> SNISRQAYADMFGPTVGDKVRLADTELWIEVEDDLTTYGEEVKFGGGKVIRDGMGQGQMLAADCVDLVLTNALIVDHWGIVKADIGVKDGRIFAIGKAGNPDIQPNVTIPIGAATEVIAAEGKIVTAGG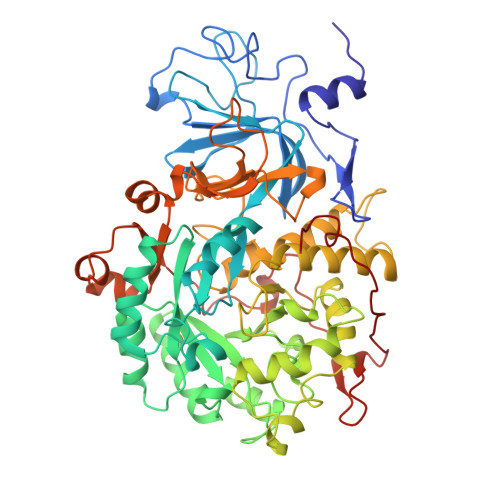IDTHIHWICPQQAEEALVSGVTTMVGGGTGPAAGTHATTCTPGPWYISRMLQAADSLPVNIGLLGKGNVSQPDALREQVAAGVIGLEIHEDWGATPAAIDCALTVADEMDIQVALHSDTLNESGFVEDTLAAIGGRTIHTFHTEGAGGGHAPDIITACAHPNILPSSTNPTLPYTLNTIDEHLDMLMVCHHLDPDIAEDVAFAESRIRRETIAAEDVLHDLGAFSLTSSDSQAMGRVGEVILRTWQVAHRMKVQRGALAEETGDNDNFRVKRYIAKYTINPALTHGIAHEVGSIEVGKLADLVVWSPAFFGVKPATVIKGGMIAIAPMGDINASIPTPQPVHYRPMFGALGSARHHCRLTFLSQAAAANGVAERLNLRSAIAVVKGCRTVQKADMVHNSLQPNITVDAQTYEVRVDGELITSEPADVLPMAQRYFLF>[2x]TRDRNGTWEMESNENFEGWMKALDIDFALRKIAVRLTQTLVIDQDGDNFKVKCTSTFWN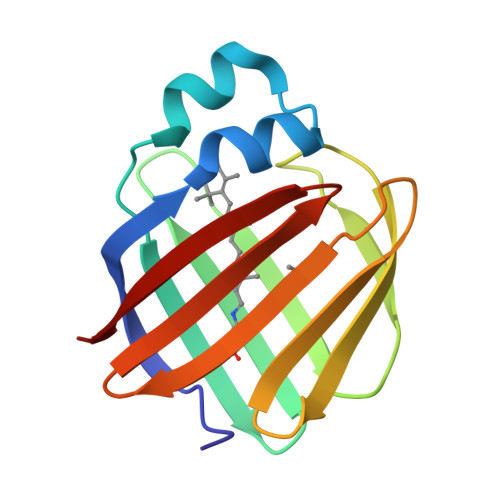YDVDFTVGVEFDEYTKSLDNRHVKALVTWEGDVLVCVQKGEKENRGWKKWIEGDKLYLELTCGDQVCRQVFKKK> GAAAMVQAWYMDDAPGDPRQPHRPDPGRPVGLEQLRRLGVLYWKLDADKYENDPELEKIRRERNYSWMDIIT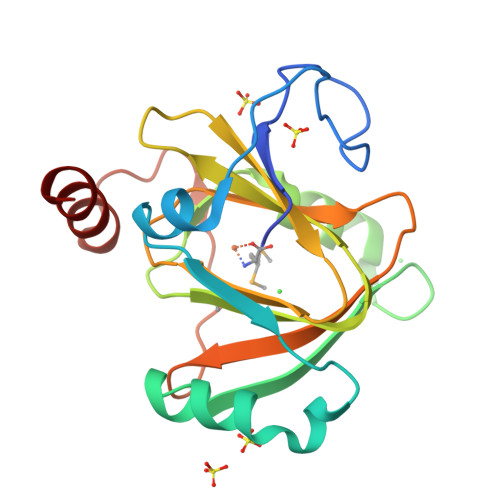ICKDKLPNYEEKIKMFYEEHLHLDDEIRYILDGSGYFDVRDKEDQWIRIFMEKGDMVTLPAGIYHRFTVDEKNYTKAMRLFVGEPVWTAYNRPADHFEARGQYVKFLAQTA>SVIL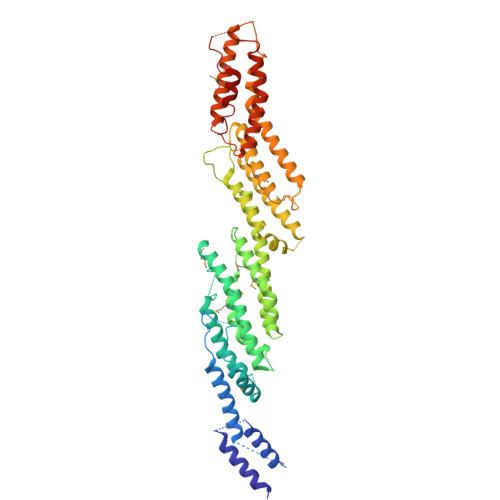SQFDLLRQAETKVLKGPHEDLESYLDAIAQLRKIIRYFMSNKSFKSSDGVLNHANSLLAKAQSKLEEEFKQLLASYSKAVEPDRLFDGLPNSLRPSSDGDGGGKPHGGHHNDDAETAAYTLPILIPSRVLPLLHDLAQQMVQAGHQQQLLQIYRDTRSFVLEESLKKLGVEKLSKEDVQRMQWEVLEAKIGNWIHFMRIAVKLLFAGERQVCDQIFRGFDSLSDQCFAEVTVSSVSMLLSFGDAIARSKRSPEKLFVLLDMYEIMRELHTEIETIFKGKACLEIRDSATGLTKRLAQTAQETFGDFEEAVEKDATKTAVLDGTVHPLTSYVINYVKFLFDYQTTLKQLFLEFGNGDDSNSQLASVTMRIMQALQNNLDGKSKQYKDPALTHLFLMNNIHYMVRSVRRSEAKDLLGDDWVQRHRRIVQQHANQYKRVAWTKILQSSSAQGLTSSGGGSLEGGNSSGVSRGLLKERFKMFNMQFDELHQRQSQWTVPDTELRESLRLAVAEVLLPAYRSFLKRFGPLVESGKNPQKYIKYTAEDLERLLGELFEGKSMNEPRR[2x]> SNRRVYKKMPSIESD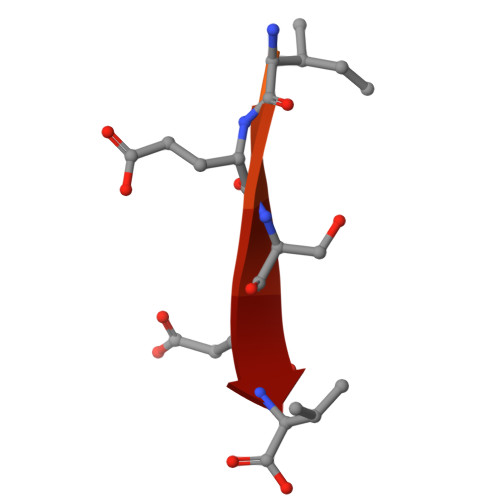V> MESKKRQWALEDFEIGRPLGKGKFGNVYLAREKQSKFILALKVLFKAQLEKAGVEHQLRREVEIQSHLRHPNILRLYGYFHDATRVYLILEYAPLGTVYRELQKLSKFDEQRTATYITELANALSYCHSKRVIHRDIKPENLLLGSAGELKIADFGWSVHAPSSRRTTLCGTLDYLPPEMIEGRMHDEKVDLWSLGVLCY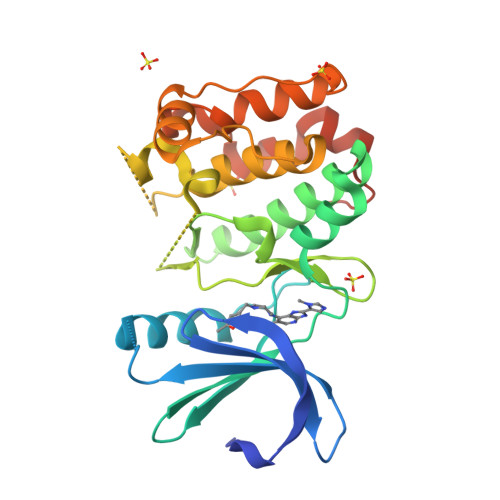EFLVGKPPFEANTYQETYKRISRVEFTFPDFVTEGARDLISRLLKHNPSQRPMLREVLEHPWITANSSKPSNCQNKESASKQS[2-[[(2~{S},3~{S},4~{S},5~{S},6~{R})-6-(hydroxymethyl)-3,4,5-tris(oxidanyl)oxan-2-yl]amino]-1,3-thiazol-5-yl]-(4-methyl-2-pyrazin-2-yl-1,3-thiazol-5-yl)methanone 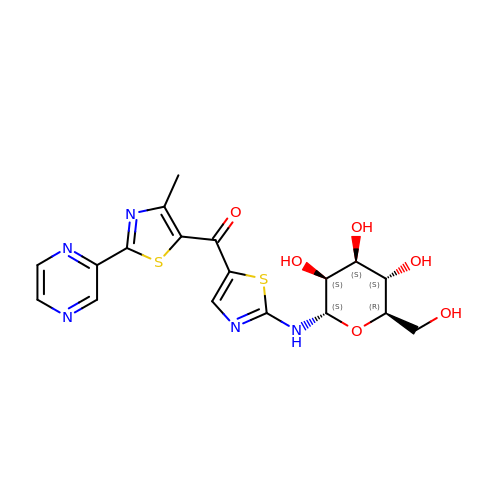| C18 H19 N5 O6 S2 | FESQRGIJCSQMRT-UFMGXSJKSA-N3-nitropyridin-2-amine | C5 H5 N3 O2 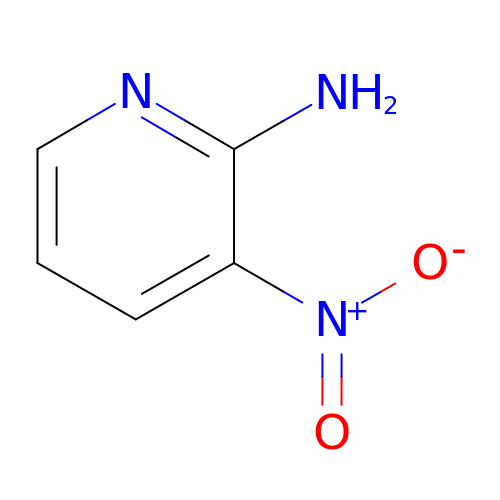| BPYHGTCRXDWOIQ-UHFFFAOYSA-N>[2x]ELTVGINGFGRIGRLVLRVCMEKGIRVVAVNDPFIDPEYMVYMFKYDSTHGRYKGNVEHKNGQLVVDNLEINTYQCKDPKEIPWSSIGNPYVVECTGVYLSIEAASAHISSGARRVVVTAPSPDAPMFVM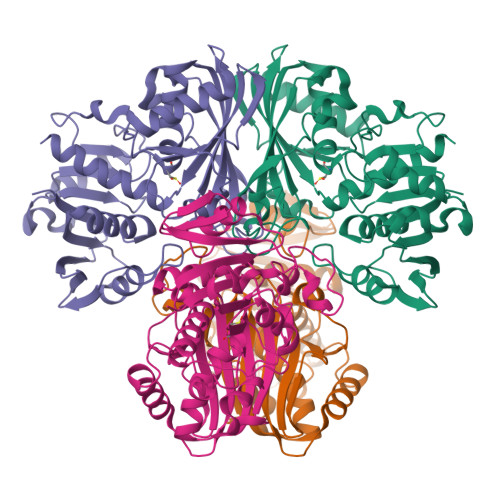GVNEKDYNPGSMTIVSNASCTTNCLAPLAKVIHENFGIVEGLMTTVHSYTATQKTVDGPSKKDWRGGRGAHQNIIPSSTGAAKAVGKVIPELKGKLTGMAFRVPTPNVSVVDLTCRLAKPASYSAITEAVKAAAKGPLAGILAYTEDQVVSTDFNGNPHSSIFDAKAGIALNDNFVKLVAWYDNEYGYSNRVVDLLRYMFSRE> GSSMGSLNQDATILRQA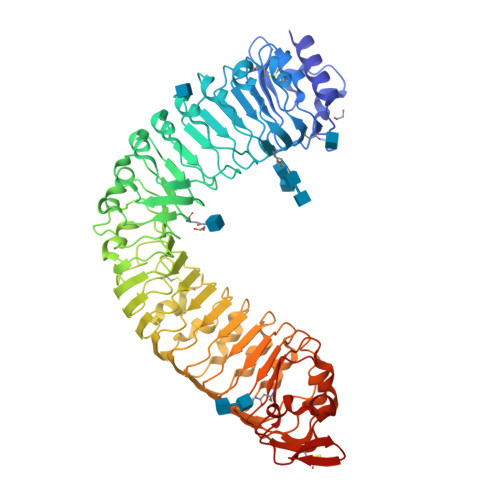KLGLSDPAQSLSSWSDNNDVTPCKWLGVSCDATSNVVSVDLSSFMLVGPFPSILCHLPSLHSLSLYNNSINGSLSADDFDTCHNLISLDLSENLLVGSIPKSLPFNLPNLKFLEISGNNLSDTIPSSFGEFRKLESLNLAGNFLSGTIPASLGNVTTLKELKLAYNLFSPSQIPSQLGNLTELQVLWLAGCNLVGPIPPSLSRLTSLVNLDLTFNQLTGSIPSWITQLKTVEQIELFNNSFSGELPESMGNMTTLKRFDASMNKLTGKIPDNLNLLNLESLNLFENMLEGPLPESITRSKTLSELKLFNNRLTGVLPSQLGANSPLQYVDLSYNRFSGEIPANVCGEGKLEYLILIDNSFSGEISNNLGKCKSLTRVRLSNNKLSGQIPHGFWGLPRLSLLELSDNSFTGSIPKTIIGAKNLSNLRISKNRFSGSIPNEIGSLNGIIEISGAENDFSGEIPESLVKLKQLSRLDLSKNQLSGEIPRELRGWKNLNELNLANNHLSGEIPKEVGILPVLNYLDLSSNQFSGEIPLELQNLKLNVLNLSYNHLSGKIPPLYANKIYAHDFIGNPGLCVDLDGLCRKITRSKLEGSENLYFQ> GSG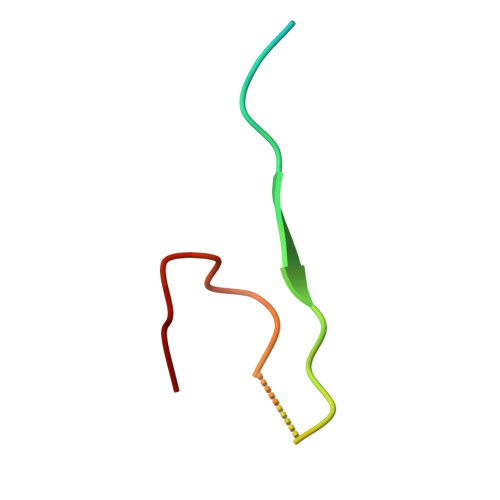AGEAEERVVVIDDDEDDDAENSSSRY>MSTKVKKTTQLKQMLNSKDLEFIMEAHNGLSARIVQEAGFKGIWGSGLSVSAQLGVRASNEASWTQVVEVLEFMSDASDVPILLDADTGYGNFNNARRLVRKLEDRGVAGACLEDKLFPKTNSLHDGRAQPLADIEEFALKIKACKDSQTDPDFCIVARVEAFIAGWGLDEALKRAEAYRNAGADAILMHSKKADPSDIEAFMKAWNNQGPVVIVPTKYYKTPTDHFRDMGVSMV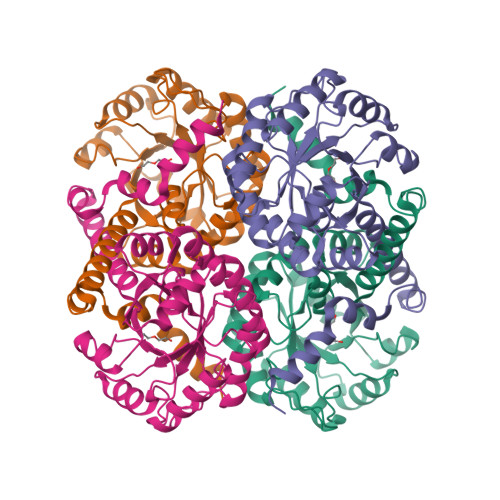IWANHNLRASVSAIQQTTKQIYDDQSLVNVEDKIVSVKEIFRLQRDDELVQAEDKYLPKN[2x]>[2x]MDYKDDDDKAAYDNQTIGRGETSKSMHLSAGDTAKNTTINSGGKQYVSSGGSATSTTINIGGVQHVSSGGSATSSTINSGGHQHVSSGGSATNTTVNNGGRQTVFSGGSAMGTIINSGGDQYVISGGSATSA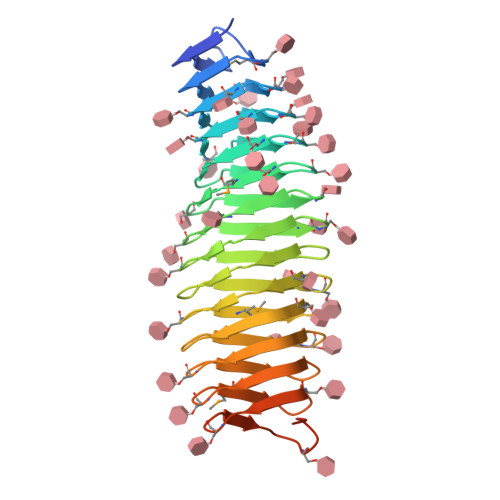SVTSGARQFVSSGGIVKATSVNSGGRQYVRDGGSATDTVLNNTGRQFVSSGGSAAKTTINSGGGMYLYGGSATGTSIYNGGRQYVSSGGSATNTTVYSGGRQHVYIDGNVTETTITSGGMLQVEAGGSASKVIQNSGGAVITNTSAAVSGTNDNGSFSIAGGSAVNMLLENGG>CG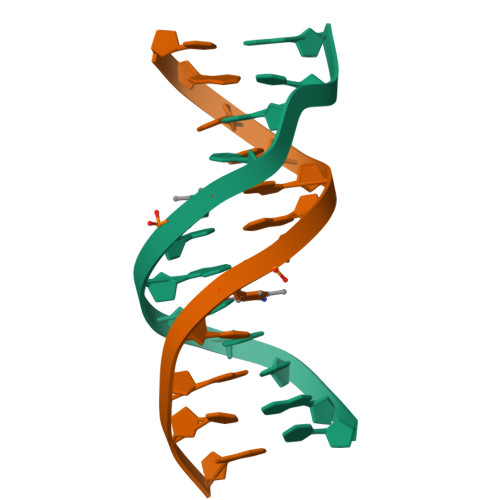CAIATCTGCG[2x]>MRGSHHHHHHGSMVLGKPQTDPTLEWFLSHCHIHKYPSKSTLIHQGEKAETLYYIVKGSVAVLIKDEEGKEMILSYLNQGDFIGELGLFEEGQERSAWVRAKTACEVAEISYKKFRQLIQVNPDILMRLSAQMARRLQVTSEKVGNLAFLDVTGRIAQTLLNLAKQPDAMTLPDGMQIKITRQEIGQIVGCSRETVGRILKMLEDQNLISAHGKTIVVYGTR[2x]

CAP is a 210-amino-acid transcription factor that binds cAMP generated by adenylyl cyclase in response to the phosphorylated form of Enzyme IIAGlc (phosphorylated in response to the phosphoenolpyruvate-carbohydrate phosphotransferase system). cAMP-bound CAP regulates the transcription of over 100 genes crucial for carbon utilization through its binding to a specific promoter region and recruitment of RNA polymerase. Previous studies of the ligand binding domain of CAP demonstrated negative cooperativity between cAMP binding sites in the absence of structural change within this domain. We produce coarse-grained models that describe global low-frequency protein backbone motions of CAP and show a strong correlation between negative cooperativity for cAMP and modulation of the delocalised normal modes on ligand binding without a requirement for a spatially distinct physical pathway or conformational change. We demonstrate experimentally that altered connectivity between backbone elements in CAP can give predictable alterations to cooperativity for cAMP binding through altered mode amplitudes.

We examined amino acids predicted to show altered (V132, H160) or neutral (V140) responses to altered amino acid side chain interactions. The ENM calculations predicted a reduction in the negative cooperativity of CAP in response to a reduction in the strength of the local interactions of residue H160. In particular, H160 was predicted to form interactions that contribute to allostery with D162 and Q165. The mutation H160L was predicted to break these interactions while maintaining side chain bulk; this was confirmed by X-ray crystallography of the H160L CAP protein. No overall change in H160L protein structure was evident compared to wild-type. ITC experiments demonstrated that cooperativity for cAMP became less negative as predicted by computation. This crucial experiment demonstrates that altering low-frequency motions at a site distant from both the ligand binding site as well as the dimer interface, and from any presumed physical pathway of structural change connecting these sites, can nonetheless give predictable effects on cooperativity.>[4x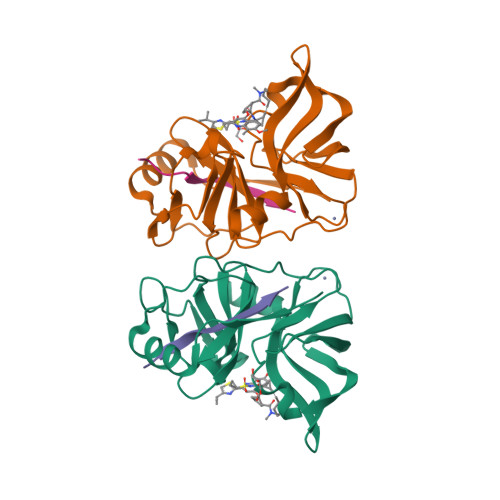]MAPITAYSQQTRGLLGCIITSLTGRDKNQVEGEVQVVSTATQSFLATCVNGVCWTVYHGAGSKTLAGPKGPITQMYTNVDQDLVGWQAPPGARSLTPCTCGSSDLYLVTRHADVIPVRRRGDSRGSLLSPRPVSYLKGSSGGPLLCPSGHAVGIFRAAVCTRGVAKAVDFVPVESMETTMRSGSHHHHHH;>KKGSVVIVGRIVLSGKPAIIPKK[4x]The crystal structure of the Lysobacter capsici VKM B−2533T β-lytic protease (Blp), a medicinally promising antimicrobial enzyme, was first solved. Blp is known to belong to the M23 family of metalloproteases. In the peptidoglycan of target cells, the enzyme digests the bonds in the interpeptide bridge. Apart from hydrolysing substrates for proteases, the enzyme is highly efficient in digesting the peptidoglycan of living Micrococcus luteus Ac−2230T and Staphylococcus aureus 55 MRSA cells.

The Blp structure was determined at a resolution of 1.57 Å by the molecular replacement technique. The analysis revealed that the Blp structure had a folding characteristic of the M23 family proteases, the LAS superfamily. Comparative structural analysis of LasA and Blp showed a high degree of structural homology (rmsd = 1.07 Å) despite the low (44%) amino acid sequence identity of the mature parts of these proteins. The active sites of LasA and Blp were almost the same and represented a groove, the walls of which were formed mainly by four loops (1–4) and the bottom by antiparallel β−sheets (β3–β4–β5–β7–β2). The active site of Blp contained a five−coordinate zinc ion by conserved His 22, His 123, Asp 36, and formic acid, which was replaced by Wat1 and Wat2 in the LasA structure. A comparative analysis of the structures shows that a ligand, formic acid, was located at the place of these water molecules in the Blp structure. Sodium acetate, which was used in the isolation and crystallization of the protein, contained a formate impurity. The C−terminal subdomain and disulphide bridge Cys156–Cys169 were preserved in the Blp structure. The conformational lability of the Cys112 side group in the Blp structure was implemented in two positions, one of which did not form the cysteine bridge in 41% of cases. Access to the LasA active site was more restricted than the Blp active site due to the bulky charged side groups Arg60, Arg68, Trp41, and Asn20.

> SPNGLLQFPFPRGARWHVGGAHTNTGSGNYPMSSLDMSLGGGWGSNQSGTWVSASAAGSFKRHSSCFAEVVHSGGWSTTYYHLMNIQYNTGANVSMNTAIANPANTQAQALCNGGSSTGPHEHWSLKQNGSFYHLNGTYLSGYRITATGSSYDTNCSRFYLTKNGQNYCYGYYTNPGPN> MFLGIRDIRAAAGRFALIASVVGLITLLIVMLTGLTQGLGKQNTSAIEALAPHSVVFTTAGGSSPEFTSSEISEQQAERWKDSTPLGVSQTRIESDQNANTTAVMGLPEGTPLPDSVGGFIEQGA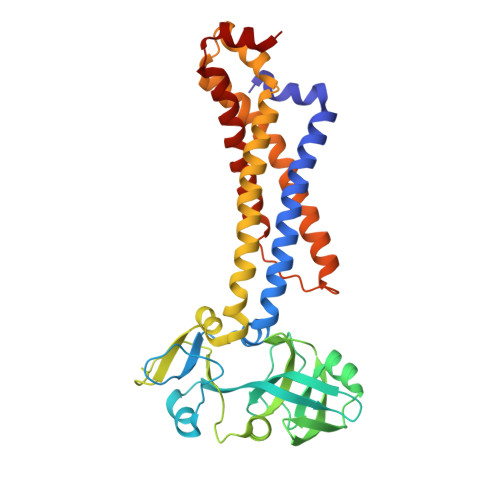LLPAELADFLHVRAGDHITLGGATVTVAGTVKTENYSHTPVVWVDTATWQLVSHTKAVGTVLLLNQEPTIQPQDNEVVTDLKGAFQAMPAYKSERSSLLSMQAFLYIISALVTVAFLTVWTLQRTRDIAVLAALGASKRYLLIDALGQAAIILAAGVALGAGIGALLGWLIAGSVPFSLGWVSVLGPALGIWLLGLIGATIAVRNVTKVDPQIALGATA>[2x]MSNMKKDTNEIVQDLKKILGIVSLIKSANNEHQAYKILMENNSFIIRTINKVLADSNYIIKIIALFNTDVVSDKIKLEEYKDVFSFSKENVIFGIKCFCDITIDGIDQINNKYVSFFKKVLPNIILFQTSCVKTTQFVNIFSKLSSIVYSEILTNE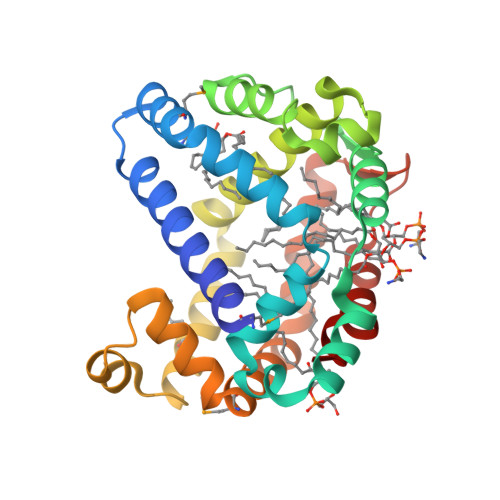RLHVLFSEIMASFKTKVSVEDLKKRKVNNIQGLISEISNNREMYKNIFVEEYEKHKTTLISIVQCITDNYNINYKENAVDIEFIFDFIQEHYISKL>MQLNVRSTASGARSSTRSRRMTAVVQAVAQRAGTIDVQRNENFGKLRAGYLFPEIARRRKAHQEKNPDAKIISLGIGDTTEPLPKYIADAMAKAAAGLATREGYSGYGAEQGQGALREAVASTFYGHAGRAADEIFISDGSKCDIARIQMMFGSKPTVAVQDPSYPVYVDTSVMMGMTGDHNGTGFDGIEYMVCNPDNHFFPDLSKAKRTDIIFFCSPNNPTGAAATRAQLTELVNFARKNGSILVYDAAYALYISNPDCPKTIYEIPGADEVAIETCSFSKYAGFTGVRLGWTVVPKALKYANGEPVHADWNRVMTTCFNGASNIVQAGGLACLQPEGLKEMNAMIKFYKENAQILKTTFTEMGFSVYGGDDAPYIWVGFPGKPSWDVFAEILERCNIVTTPGSGYGPAGEGFVRASAFGSRENILEAVRRFKEAYGKRNASHHHHHH[2x]

The DAP/lys pathway can be divided into three parts. three steps that bypassed by the reaction catalyzed by DapL. as a pyridoxal phosphate (PLP)-dependent transferase-like fold by SCOP. enzyme, the algal enzyme is specific for L,L-DAP.

Cr-DapL is a dimer in solution. demonstrating that the enzyme DapL is dimeric in solution. The predicted mass of the dimer is 97.66 kDa. two monomers in the asymmetric unit. V-shaped monomer and comprises residues from both monomers in the dimer. residues that are contributed from the opposing monomer in the dimer. Numbering is based on the Cr-DapL structure. substrate recognition, fills the space that would be taken by the PLP cofactor. active site does not easily fit the cyclic THDPA species. strain expressing the algal enzyme is able to grow on DAP-free media.>SNHHRGLASANVDFAFSLYKHLVALSPKKNIFISPVSISMALAMLSLGTCGHTRAQLLQGLGFNLTERSETEIHQGFQHLHQLFAKSDTSLEMTMGNALFLDGSLELLESFSADIKHYYESEVLAMNFQDWATASRQINSYVKNKTQGKIVDLFSGLDSPAILVLVNYIFFKGTWTQPFDLASTREENFYVDETTVVKVPMMLQSSTISYLHDSELPCQLVQMNYVGNGTVFFILPDKGKMNTVIAALSRDTINRWSAGLTSSQVDLYIPKVTISGVYDLGDVLEEMGIADLFTTQANFSR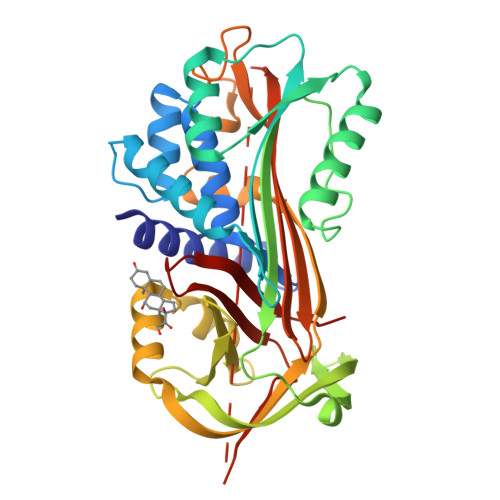ITQDAQLKSSKVVHKAVLQLNEEGTEAAGAMFLEAIPRSKPIILRFNQPFIIMIFDHFTWSSLFLARVMNPV[2x]> MAMSNGNNDFVVLSNSSIATSAANPSPLTPCDGDHAAQQLTPKEATRTKVSPNGCLQLNGTVKSSFLPLDNQRMPQMLPQCCHPCPYHHPLTSHSSHQECHPEAGPAAPSALASCCMQPHSEYSASLCPNHSPVYQTTCCLQPSPSFCLHHPWPDHFQHQPVQQHIANIRPSRPFKLPKSYAALIADWPVVVLGMCTMFIVVCALVGVLVPELPDFSDPLLGFEPRGTAIGQRLVTWNNMVKNTGYKATLANYPFKYADEQAKSHRDDRWSDDHYEREKREVDWNFHKDSFFCDVPSDRYSRVVFTSSGGETLWNLPAIKSMCNVDNSRIRSHPQFGDLCQRTTAASCCPSWTLGNYIAILNNRSSCQKIVERDVSHTLKLLRTCAKHYQNGTLGPDCWDMAARRKDQLKCTNVPRKCTKYNAVYQILHYLVDKDFMTPKTADYATPALKYSMLFSPTEKGESMMNIYLDNFENWNSSDGVTTITGIEFGIKHSLFQDYLLMDTVYPAIAIVIVLLVMCVYTKSMFITLMTMFAIISSLIVSYFLYRVVFHFEFFPFMNLTALIILVGIGANNAFVLCDVWNYTKFDKPHAETSETVSITLQHAALSMFVTSFTTAAAFYANYVSNITAIRCFGVYAGTAILVNYVLMVTWLPAVVVLHERYLLNIFTCFKKPQQQIYDNKSCWTVACQKCHKVLFAISEASRIFFEKVLPCIVIKFRYLWLFWFLALTVGGAYIVCINPKMKLPSLELSEFQVFRSSHPFERYDAEYKKLFMFERVHHGEELHMPITVIWGVSPEDNGNPLNPKSKGKLTLDSSFNIASPASQAWILHFCQKLRNQTFFYQTDEQDFTSCFIETFKQWMENQDCDEPALYPCCSHWSFPYKQEIFELCIKRAIMELERSTGYHLDSKTPGPRFDINDTIRAVVLEFQSTYLFTLAYEKMHQFYKEVDSWISSELSSAPEGLSNGWFVSNLEFYDLQDSLSDGTLIAMGLSVAVAFSVMLLTTWNIIISLYAIISIAGTIFVTVGSLVLLGWELNVLESVTISVAVGLSVNFAVHYGVAYRLAPDPDREGKVIFSLSRVGSAMAMAALTTFVAGAMMMPSTVLAYTQLGTFMMLIMCISWAFATFFFQCMCRCLGPQGTCGQIPLPKKLQCSAFSHALSTSPSDKGQSKTHTINAYHLDPRGPKSELEHEFYELEPLASHSCTAPEKTTYEETHICSEFFNSQAKNLGMPVHAAYNSELSKSTESDAGSALLQPPLEQHTVCHFFSLNQRCSCPDAYKHLNYGPHSCQQMGDCLCHQCSPTTSSFVQIQNGVAPLKATHQAVEGFVHPITHIHHCPCLQGRV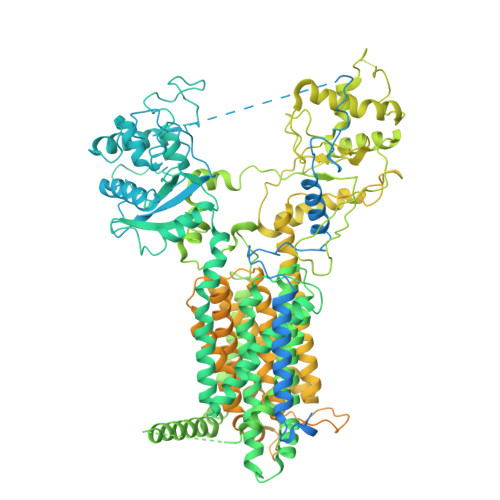KPAGMQNSLPRNFFLHPVQHIQAQEKIGKTNVHSLQRSIEEHLPKMAEPSSFVCRSTGSLLKTCCDPENKQRELCKNRDVSNLESSGGTENKAGGKVELSLSQTDASVNSEHFNQNEPKVLFNHLMGEAGCRSCPNNSQSCGRIVRVKCNSVDCQMPNMEANVPAVLTHSELSGESLLIKTL> SVERVYQKKTQLEHILLRPDTYIGSVEPLTQFMWVYDEDVGMNCREVTFVPGLYKIFDEILVNAADNKQRDKNMTCIKVSIDPESNIISIWNNGKGIPVVEHKVEKVYVPALIFGQLLTSSNYDDDEKKVTGGRNGYGAKLCNIFSTKFTVETACKEYKHSFKQTWMNNMMKTSEAKIKHFDGEDYTCITFQPDLSKFKMEKLDKDIVALMTRRAYDLAGSCRGVKVMFNGKKLPVNGFRSYVDLYVKDKLDETGVALKVIHELANERWDVCLTLSEKGFQQISFVNSIATTKGGRHVDYVVDQVVGKLIEVVKKKNKAGVS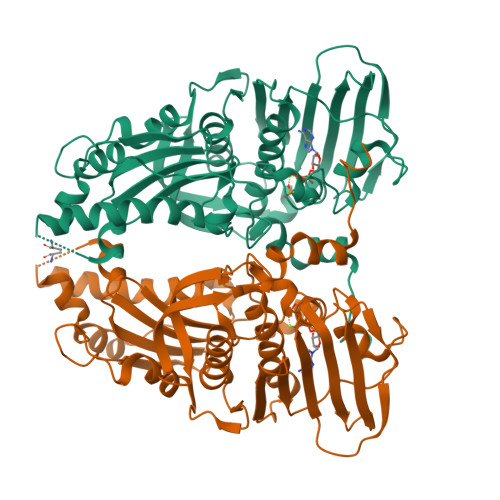VKPFQVKNHIWVFINCLIENPTFDSQTKENMTLQPKSFGSKCQLSEKFFKAASNCGIVESILNWVKFKAQTQLNKKCS> LKESPSGYLRSGEGDTGCGELVWVGEPLTLRTAETITGKYGVWMRDPKPTYPYTQETTWRIDTVGKDVRQVFEYDLISQFMQGYPSKVHILPRPLESTGAVVYSGSLYFQGAESRTVIRYELNTETVKAEKEIPGAGYHGQFPYSWGGYTDIDLAVDEAGLWVIYSTDEAKGAIVLSKLNPENLELEQTWETNIRKQSVANAFIICGTLYTVSSYTSADATVNFAYDTGTGISKTLTIPFKNRYKYSSMIDYNPLEKKLFAWDNLNMVTYDIKLSKM

Inherited missense mutations in the myocilin (MYOC) gene, within its olfactomedin (OLF) domain, constitute the strongest genetic link to primary open-angle glaucoma via a toxic gain of function, and thus MYOC is an attractive precision-medicine target. Myocilin has no known function, and there is no glaucoma phenotype in Myoc knockout mice or in individuals with a homozygous N-terminal truncation mutation or hemizygous deletion of MYOC, but rare non-synonymous coding mutations lead to toxic intracellular sequestration of misfolded myocilin. However, not all mutations in MYOC cause glaucoma, and common variants are expected to be neutral polymorphisms. Among the common features associated with pathogenic myocilin misfolding, we demonstrate that a single metric, OLF thermal stability, can robustly segregate benign from early-onset disease variants.

At the outset of our study, five variants could be confidently predicted as benign polymorphisms: T293K, T353I, K398R, A445V and K500R. These mutations are all found on the protein surface and well documented in the literature. Thr to Lys and Thr to Ile are less conservative changes, but in prior studies, T293K and T353I exhibited wild type (WT)-like cellular secretion and WT-like thermal stability, and were found in the control group for case–control clinical studies. Modestly lower levels than WT were detected for T293K, E352K, K398R, N420Y and A427T. Structural integrity was further confirmed by high-resolution crystal structures, which were solved for 11 OLF variants. No gross changes from WT OLF were detected for the structures of T293K, R296H, L303I, V329M, S331L, E352K, T353I, K398R, A445V, V449I or K500R, indicating that these mutations are accommodated within the native five-bladed β-propeller fold and do not perturb the dinuclear calcium-containing site.> MEKDGLCRADQQYECVAEIGEGAYGKVFKARDLKNGGRFVALKRVRVQTGEEGMPLSTIREVAVLRHLETFEHPNVVRLFDVCTVSRTDRETKLTLVFEHVDQDLTTYLDKVPEPGVPTETIKDMMFQLLRGLDFLHSHR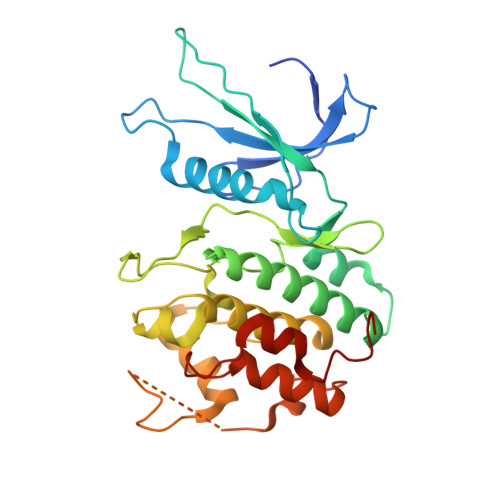VVHRDLKPQNILVTSSGQIKLADFGLARIYSFQMALTSVVVTLWYRAPEVLLQSSYATPVDLWSVGCIFAEMFRRKPLFRGSSDVDQLGKILDVIGLPGEEDWPRDVALPRQAFHSKSAQPIEKFVTDIDELGKDLLLKCLTFNPAKRISAYSALSHPYFQDLERCKE> MLRFFRARLAPTTTDAAAKLPAGNPVNKTWFRH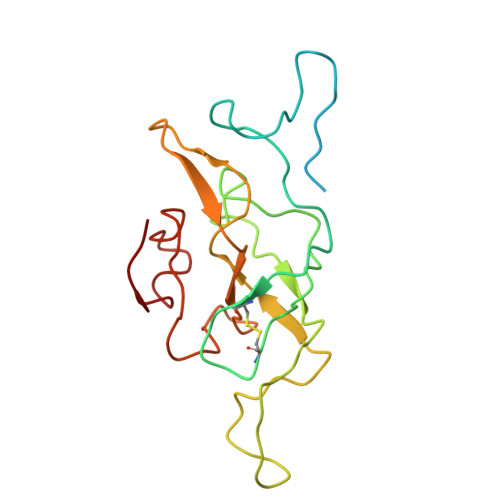NLIIRRKGSYRSRWGNGTEGYGAGVPLSDQVKLHCVDNTNCKHVRLIAKATAERFAHCRVFPAVAHRVSVQRFKGRGGGGEVSRHRVKPGNIYWVCLFTRRQTNTRMSGLQTNFDRNTCIIMNDQRVPLGTRVMYCAGRHVNHKYHLKAVVLANFFV[[(2~{S},5~{R})-5-(4-azanyl-5-fluoranyl-2-oxidanylidene-pyrimidin-1-yl)-1,3-oxathiolan-2-yl]methoxy-oxidanyl-phosphoryl] 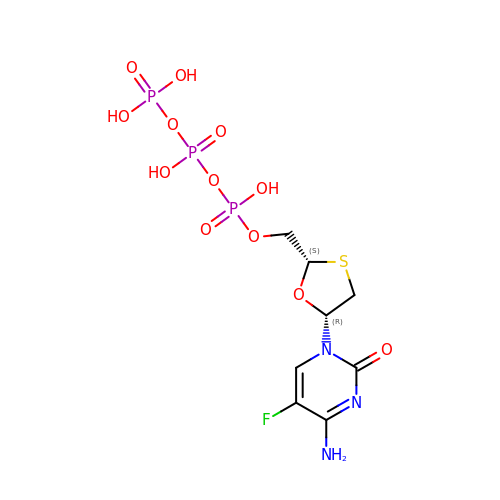phosphono hydrogen phosphate | C8 H13 F N3 O12 P3 S | WIEOLFZNMKSGEX-RITPCOANSA-N>[6x]MAGNKPFNKQQAEPRERDPQVAGLKVPPHSIEAEQSVLGGLMLDNERWDDVAERVVADDFYTRPHRHIFTEMARLQESGSPIDLITLAESLERQGQLDSVGGFAYLAELSKNTPSAANISAYADIVRERAVVREMISVANEIAEAGFDPQGRTSEDLLDLAESRVFKIAESRANKDEGPKNIADVLDATVARIEQLFQQPHDGVTGVNTGYDDLNKKTAGLQPSDLIIVAARPSMGKTTFAMNLVENAAMLQDKPVLIFSLEMPSEQIMMRSLASLSRVDQTKIRTGQLDDEDWARISG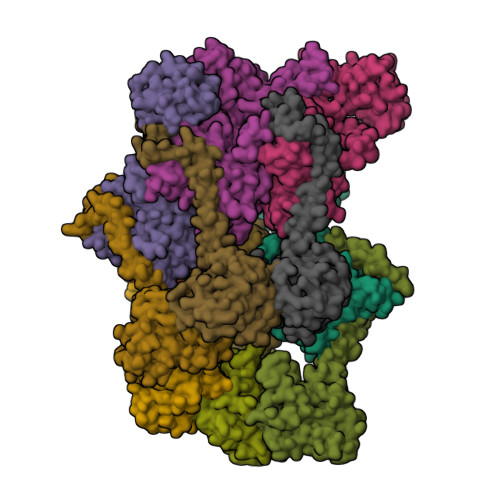TMGILLEKRNIYIDDSSGLTPTEVRSRARRIAREHGGIGLIMIDYLQLMRVPALSDNRTLEIAEISRSLKALAKELNVPVVALSQLNRSLEQRADKRPVNSDLRESGSIEQDADLIMFIYRDEVYHENSDLKGIAEIIIGKQRNGPIGTVRLTFNGQWSRFDNYAGPQYDDE;>[6x]MKNVGDLMQRLQKMMPAHIKPAFKTGEELLAWQKEQGAIRSAALERENRAMKMQRTFNRSGIRPLHQNCSFENYRVECEGQMNALSKARQYVEEFDGNIASFIFSGKPGTGKNHLAAAICNELLLRGKSVLIITVADIMSAMKDTFRNSGTSEEQLLNDLSNVDLLVIDEIGVQTESKYEKVIINQIVDRRSSSKRPTGMLTNSNMEEMTKLLGERVMDRMRLGNSLWVIFNWDSYRSRVTGKEY> MSAKAISEQTGKELLYKFICTTSAIQNRFKYARVTPDTDWARLLQDHPWLLSQNLVVKPDQLIKRRGKLGLVGVNLTLDGVKSWLKPRLGQEATVGKATGFLKNFLIEPFVPHSQAEEFYVCIYATREGDYVLFHHEGGVDVGD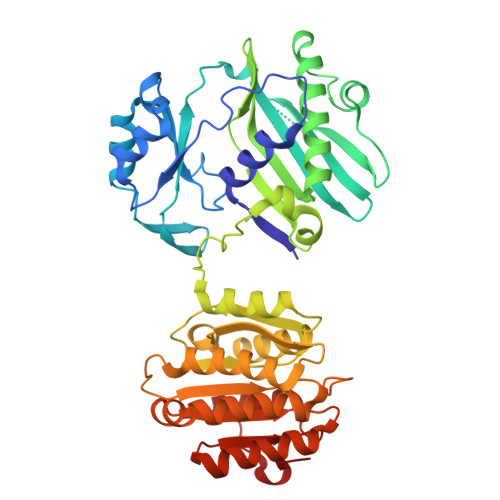VDAKAQKLLVGVDEKLNPEDIKKHLLVHAPEDKKEILASFISGLFNFYEDLYFTYLEINPLVVTKDGVYVLDLAAKVDATADYICKVKWGDIEFPPPFGREAYPEEAYIADLDAKSGASLKLTLLNPKGRIWTMVAGGGASVVYSDTICDLGGVNELANYGEYSGAPSEQQTYDYAKTILSLMTREKHPDGKILIIGGSIANFTNVAATFKGIVRAIRDYQGPLKEHEVTIFVRRGGPNYQEGLRVMGEVGKTTGIPIHVFGTETHMTAIVGMALGHRPIPENLYFQ>MKEFYLTVEQIGDSIFERYIDSNGRERTREVEYKPSLFAHCPESQATKYFDIYGKPCTRKLFANMRDASQWIKRMEDIGLEALGMDDFKLAYLSDTYNYEIKYDHTKIRVANFDIEVTSPDGFPEPSQAKHPIDAITHYDSIDDRFYVFDLLNSPYGNVEEWSIEIAAKLQEQGGDEVPSEIIDKIIYMPFDNEKELLMEYLNFWQQKTPVILTGWNVESFAIPYVYNRIKNIFGESTAKRLSPHRKTRVKVIENMYGSREIITLFGISVLDYIDLYKKFSFTNQPSYSLDYISEFELNVGKLKYDGPISKLRESNHQRYISYNIIAVYRVLQIDAKRQFINLSLDMGYYAKIQIQSVFSPIKTWDAII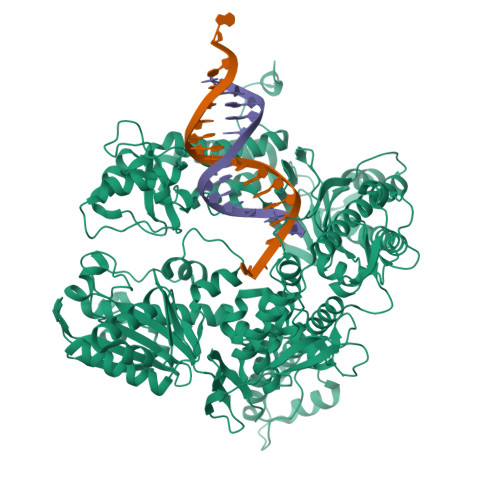FNSLKEQNKVIPQGRSHPVQPYPGAFVKEPIPNRYKYVMSFDLTSLYPSIIRQVNISPETIAGTFKVAPLHDYINAVAERPSDVYSCSPNGMMYYKDRDGVVPTEITKVFNQRKEHKGYMLAAQRNGEIIKEALHNPNLSVDEPLDVDYRFDFSDEIKEKIKKLSAKSLNEMLFRAQRTEVAGMTAQINRKLLINSLYGALGNVWFRYYDLRNATAITTFGQMALQWIERKVNEYLNEVCGTEGEAFVLYGDTDSIYVSADKIIDKVGESKFRDTNHWVDFLDKFARERMEPAIDRGFREMCEYMNNKQHLMFMDREAIAGPPLGSKGIGGFWTGKKRYALNVWDMEGTRYAEPKLKIMGLETQKSSTPKAVQKALKECIRRMLQEGEESLQEYFKEFEKEFRQLNYISIASVSSANNIAKYDVGGFPGPKCPFHIRGILTYNRAIKGNIDAPQVVEGEKVYVLPLREGNPFGDKCIAWPSGTEITDLIKDDVLHWMDYTVLLEKTFIKPLEGFTSAAKLDYEKKASLFDMFDFHHH[2x]>[7x]MANTDYAGNLTRPHWGGAASDVDIHLEVYQNEVDTRFQYQAMFLGLSSQRSVADRSNTYRIDRLNTSSVKGRTSGVALEPTPVRNDKMLIVVDTVLYIRNPIDYQDDWTAPDFLTEMGQNNGSEFAEVFDQAHLIQLIKGRSWVAPAHLKPAFSDGIEIEATIDSDVTTQAGMEANAIAINQAHKAGIDELIKRKVPLNDMITLVSTEIYSLLLEHPKLFNKDWGDANANGYKERRAVLMNGIPVVECTEFPDAGTHPLGSAYTVTADDAKCRMVTFSKSRTLVTVEAKPFTSRIWDDEQNFANVLDCYAMYQVGERRPDTAAVVKFNEAP;>MAVAKATAAQRQEFLRQLNILAKDMYQALTQPQDLAYRGPEIDAKIAALEAATAAVKAAS[4x];>[2x]MASIIAAKAKDKQYEIVGKAQNLLKQVQPLYNVGFSTTALDLLNAYF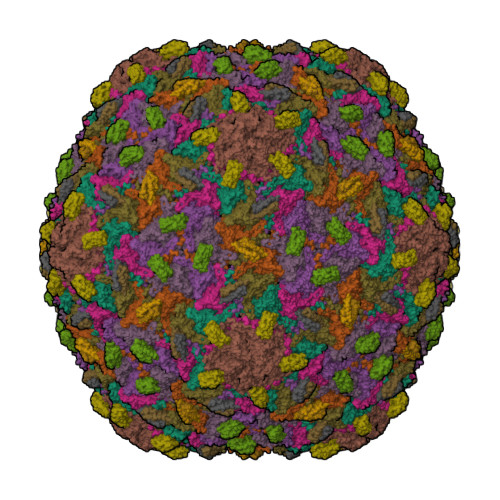TYMQAQGFATTRAGTGFVSDGAKLARLDNMLDQVSKTGYVVLTGTGAPIGETSGTAFDTSFTALRAAFLAATTPTTA>[2x]MHSTNNNSNKRNNEEKHKQPEIDSSANNGEGTSGTRAQTVGDTATEAGVRNETEAGASTRRQTDGTGLSGTNAKIATASSARQADVEKPADVTFTIENVDDVGIMQQKKPPTVVQSRTDVFNEQFANEALHPTTKVIFNGLDVNTEVQPLSDDFKQISDPKGYLTYSVKYEDQFTKKDKLRASEADDRIVGPTVNLFKYGAAVVNIDLNRDFFDTATGIDLTKGIPLVQDLLVPIGVTAGAEQSAEYVSGLLMVLFKVMTDNRLVIVGETTTPMSNTLSTVVNNVLRTTYHNNVGVNPALLRDFTQVNWLNRDITNMLQQAGTKYGLGLTETRLDYVRLVKTIVGHALNIDHFAASVLNINLRALMEANVTADDRIKALQAHSMISTQFHGPNQGALRPELAFDHDHIIRCLMLAAANYPRLEGIIVQINTGYVASANVIRPVSEKRYFPENLEQNQSAARLVSAVKARASEADISSIHLAIAREVSPMFNVHELKKIAESFEDPSSIVVVLEFILFALFFPTEFNRIKGDIQNVLLLFFSRWYPVEYGIFVQRGATYTINAAGEFEFSGRNEKWDQALYLSEHFPALFSDVPLAGANTIIAIMRLFTPQGFLRTDDLAIAANFPRASRNPQTYIPYTNQRGTVTNEFASRFRTIVATLANVVNERAVQDDMQKATRSCTKQWLRHLETQFDNIAVAHTDHLSVVYATMSNFMLNFTNNFSGNHATFKPDQYVITSPEGSYKPIIERQGETVDGLTIIDTSIVWPILCQCTYPLVRQSGKGVDAVSIMEEIVYPDPSTTLSQSLSVAQVLSKLTLPDAFINMILSGGDSVVMRTYQTEADDDLDEGIRMTTYDQYLSHIRERLHITNVPDPIYITGASTPDQIAASVQATHVAVVLYQSGVINGPASTYLRENEVLVVMPDYYDVVSRFANANLQMNNNRYHESVLEIADIFDQADFIQTSDAVRQLRALMPTLSTSQIRHAIERIAQITDVDSTDYGKLTLRFLGTLTRSLKMQNAQIRRIRPDGTVLRYDDQIDIEAFRWSRYFLDELQLRRLSVGLRLITNPRIARRFNGVRIMYLTDDDPDPDFVPDVPEGYVAVQYAHRLFSSSLANKRNRVTYTHPPTGMAYPSPTGRPHVHMTINERAGMSKLVADNIIASVIKSNWVVDILDIEYTAEVMTPSEGYTQHVDAESIMTAPKGKLFHLQFMDGLLRPEPSAFDPPASGEDMRLIYPLQPISVARSMRAIVNHNEVDRPRGAVAPSSYEMDTGTLSRNGDLLYSPVANGQVGIPKLEVDHISFSNVVSMMTANIRTGDDMAVERVNPDDVRAINIRNA;> MWHYTSINNDTRVALDPKPNQIRTITKPNTVPQLGTDYLYTFNSQRRSHTLRLLGPFQYFNFSETDRGHPLFRLPLKYPSKAIPADELIDNLHSWMRSVHLLHVRSEDNTLRYNWMLGVYARSTNYTTPVGQLVVNAPAILNYSNPQDAFNSVFVALGIDYIDIPITNSNIFDDSSTPYNVRIWHAPTMTEVNHILALMRKSTLVSTHSSWHWDVLHTFHYRSESDMIDHFAAKILEDWRQKEKLDKGALVEADRVVQRLIPLSSSTYVQRLAAIGALYPNEFTENVLDLSRLSTALLQLSDTYYQHANDQLRRLYRRMYNDSRTLYMTQRHQELLLAQITADPNILLYPYTYIFTTAYTS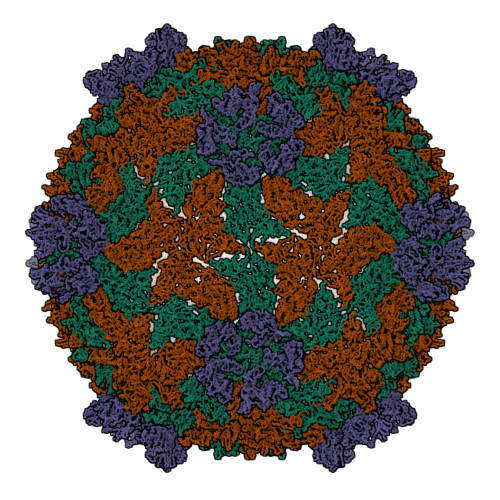MNYISNTGQGRIKHSLAVTGTTEHTIADITLGPMSEDVVTISMVEPMSIAAEDMYGYVLDTPTRDIWPADEQIEQKGDAVALYDTKTSRALGMFNNTVRIDDLLSPLLGLVYRTYIKGDTMTMTQGSLDHLTLCAAVDSDITFVGNRMIAPLAEGYIPKAMHRNNSTMKMLSLYVALKKLENFTTNSYLMAPDTSIILLGAEREPAVSILRRFNRSVSNVRIIGMGDRAVEPNIRVRVPFPIDKNISADFIICDINSYEDQSFESMFGETISVVTTCASAATRVLVKINHPSEYMINSVIERLSQLGGVFYHTALLKTASQNPYSYETYIYITPIAAAVRFPFYSNSAIINRYMTAVADDETPIIPSIHTVIKGHSNTYSPGLFCGCIDVQSAPFALSQLKSYCSEATTWRVDSDDNLVNIIARIDPARIALEFRTRSNTSAYHEYQRYVPNGLGFKGRKTREFRYIHREVTFIHKLMTYALIREQISLTENMTQVVSIGGRNLADISVVPLNMKYVVIDPATRIETLTQEKKNIEVQSRPFSFDAASMDLENNSIYLFIAVIMNEPNGAATPARTQMDKIRNVATAMLTRTNCVAYISFYEAGIITRLDQSTAHKTIRVEEGRLKVANYVPVDTLVEADVTLMLRDIGITHEIIRPSTPELINACSNYGIRLGSTGGAVLDVFNHYSPVIKLVRS>MELYLDTSDVVAVKALSRIFPLAGVTTNPSIIAAGKKPLDVVLPQLHEAMGGQGRLFAQVMATTAEGMVNDALKLRSIIADIVVKVPVTAEGLAAIKMLKAEGIPTLGTAVYGAAQGLLSALAGAEYVAPYVNRIDAQGGSGI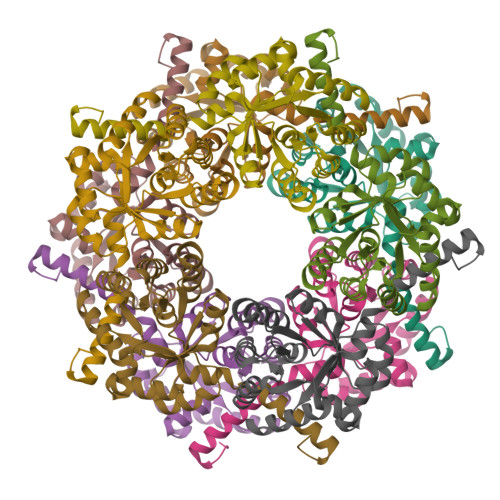QTVTDLHQLLKMHAPQAKVLAASFKTPRQALDCLLAGCESITLPLDVAQQMISYPAVDAAVAKFEQDWQGAFGRTSITSHHHHH[10x]>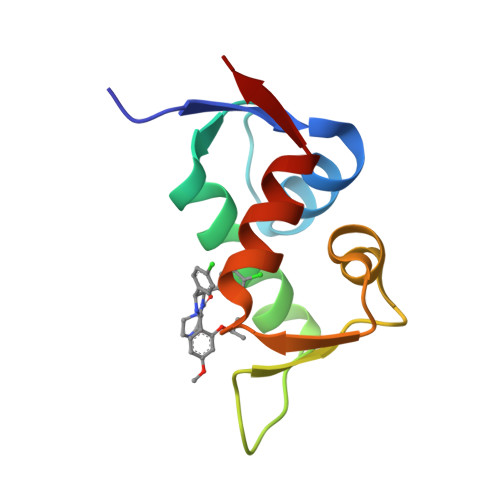 QETLVRPKPLLLKLLKSVGAQKDTYTMKEVLFYLGQYIMTKRLYDEKQQHIVYCSNDLLGDLFGVPSFSVKEHRKIYTMIYRNLVVV>GPHMGGSMEALIPVINKLQDVFNTVGADIIQLPQIVVVGTQSSGKSSVLESLVGRDLLPRGTGIVTRRPLILQLVHVSQEDKRKTTGEENGVEAEEWGKFLHTKNKLYTDFDEIRQEIENETERISGNNKGVSPEPIHLKIFSPNVVNLTLVDLPGMTKVPVGDQPKDIELQIRELILRFISNPNSIILAVTAANTDMATSEALKISREVDPDGRRTLAVITKLDLMDAGTDAMDVLMGRVIPVKLGIIGVVNRSQLDINNKKSVTDSIRDEYAFLQKKYPSLANRNGTKYLARTLNRLLMHHIRDCLPELKTRINVLAAQYQSLLNSYGEPVDDKSATLLQLITKFATEYCNTIEGTAKYIETSELCGGARICYIFHETFGRTLESVDPLGGLNTIDILTAIRNATGPRPALFVPEVSFELLVKRQIKRLEEPSLRCVELVHEEMQRIIQHCSNYSTQELLRFPKLHDAIVEVVTCLLRKRLPVTNEMVHNLVAIELAYINTKHPDFADACGLMNNNIEEQRRNRLARELPSAVSRDKSSKVPSALAPASQEPSPAASAEADGKLIQDSRRETKNVASGGGGVGDGVQEPTTGNWRGMLKTSKAEEL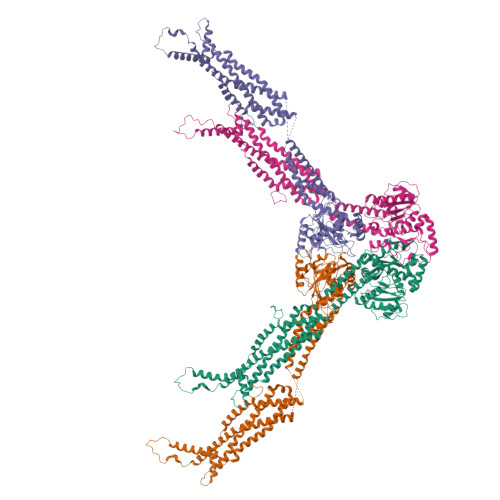LAEEKSKPIPIMPASPQKGHAVNLLDVPVPVARKLSAREQRDCEVIERLIKSYFLIVRKNIQDSVPKAVMHFLVNHVKDTLQSELVGQLYKSSLLDDLLTESEDMAQRRKEAADMLKALQGASQIIAEIRETHLW[4x]>[4x]AHMDRIIEKLDHGWWVVSHEQKLWLPKGELPYGEAANFDLVGQRALQIGEWQGEPVWLVQQQRRHDMGSVRQVIDLDVGLFQLAGRGVQLAEFYRSHKYCGYCGHEMYPSKTEWAMLCSHCRERYYPQIAPCIIVAIRRDDSILLAQHTRHRNGVHTVLAGFVEVG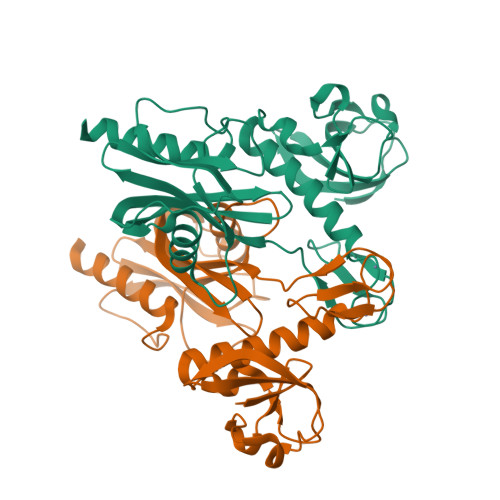ETLEQAVAREVMEQSGIKVKNLRYVTSQPWPFPQSLMTAFMAEYDSGDIVIDPKELLEANWYRYDDLPLLPPPGTVARRLIEDTVAMCRAEYE> DPDQFRAIIESPEGAGHVGYQYRRNTGSTMRMVSDVLDERVSLWDFHCDPSGNVIQPGPNVDSRQYLQAAIDYVSSNGGGTITIPAGYTWYLGSYGVGGIAGHSGIIQLRSNVNLNIEGRIHLSPFFDLKPFQVFVGFDNGDPASSGNLENCHIYGHGVVDFGGYEFGASSQLRNGVAFGRSYNCSVTGITFQNGDVTWAITLGWNGYGSNCYVRKCRFINLVNSSVNANHSTVYVNCPYSGVESCYFSMSSSFARNIACSVELHQHDTFYRGSTVNGYCRGAYVVMHAAEAAGAGSYAYNMQVENNIAVIYGQFVILGSDVTATVSGHLNDVIVSGNIVSIGERAAFSAPFGAFIDIGPDNSGASNVQDIQRVLVTGNSFYAPANITDSAAITLRANLNGCTFIANNFDCRYMVYNAPGTTSPVVQNLVWDKSNVIGGTHANQRAGQNLFDMQFASVVNSTIEVQLSCEDLSMFSCILFPASCQLSYSKITVDSAWTKSMSNTAVFEGNQQAGANVYVSYPATVNLTSYNTQGAVPFFSTDTNYAWVTSAYSLSINE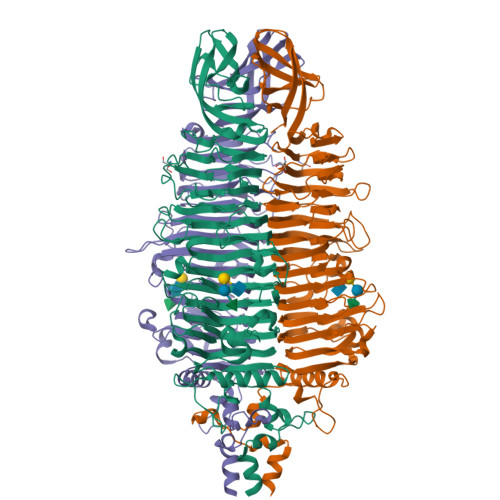NLDFSPPATYTNKANGQLVGVGYNEIGGVRSVSVRLMLQRQV> GSVWCRHCGATSAGLRCEWQNNYTQCAPCASLSSCPVCY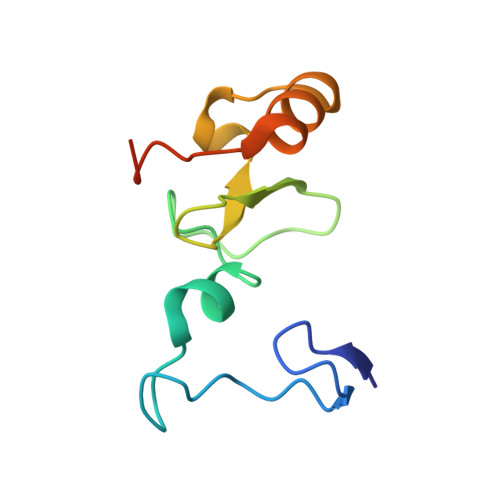RNYREEDLILQCRQCDRWMHAVCQNLNTEEEVENVADIGFDCSMCRPYMPASN>GSMRDPNFQNIDKVALLGAQPLGSSHPPGDPHAVSFSLPTWASVAGNMAGEAWVRGKKKTTYPRMGFCPIVGGLTEAALIRVKRPTGVKARIFISREAASRLEHTVKVKDPAAKVSVVQFELRQSNSPDLSNWARFVLVLFPESFEEDAFTFWLNHGDGISNRHAEFCNNLLDFMDSRCDEDEPDYQTCGPRSGDKPAGLPTWTNSGLEEKMVIKSVLAKCIRSENADMLPVQSDDVFLYSTGMMAIGKIARAMKDMPGDDTAVIFGWLYSGTLPLVKDSGYSKPILYGRGTEEELDKLESYLAAGGKCTVLFTEITSNPQLHSPNLVRIKNLADEYGFTVVVDDTIGTSVNLDILPYADVVTTSLTKIFNGACNAMGGSLIVNPNSRHYRRIHTYLQGHFEDLLFPADAVVLSENCIDYPERVKRCSATARAIAHFLAAHPSIDYVNYPTLVPSREEYERYRRDGEGYGYLLSIVFREPDFAVRFFDALDIWKGPSIGTNSSIALPYSVLAHWEEQDWAAEYGVPKHIVR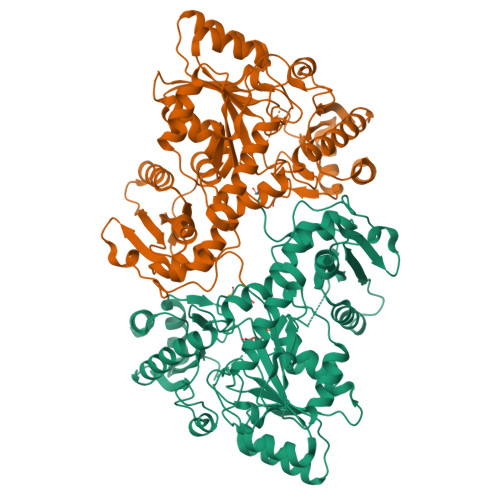LSVGLESEAWLRDRVTEALAKATPATLCRTTFCKSER[2x]>MSRLLALLALAPLLAGAAETTAPKPPSAFTVEAQRRVEAELPFADRADFERADRGLIRRPERLLIRNPDGSVAWQLGGYDFLLDGKPRDSINPSLQRQALLNLKYGLFEVAEGIYQVRGFDLANITFIRGDSGWIVVDTLTTPATARAAYELVSRELGERPIRTVIYSHAHADHFGGVRGLVEPQQVASGAVQIIAPAGFMEAAIKENVLAGNAMMRRATYQYGTQLPKGPQGQVDMAIGKGLARGPLSLLAPTRLIEGEGEDLVLDGVPFTFQNTPGTESPAEMNIWLPRQKALLMAENVVGTLHNLYTLRGAEVRDALGWSKYINQALHRFGRQAEVMFAVHNWPRWGNAEIVEVLEKQRDLYGYLHDQTLHLANQGVTIGQVHNRLRLPPSLDQEWYDRGYHGSVSHNARAVLNRYLGYYDGNPATLDPLSPEDSAGRYVEYMGGAERLLEQARASYARGEYRWVVEVVNRLVFAEPDNRAARELQADALEQLGYQAENAGWRNSYLSAAYELRHGVPRDQPTMKAGSADALAAMDTGLLFD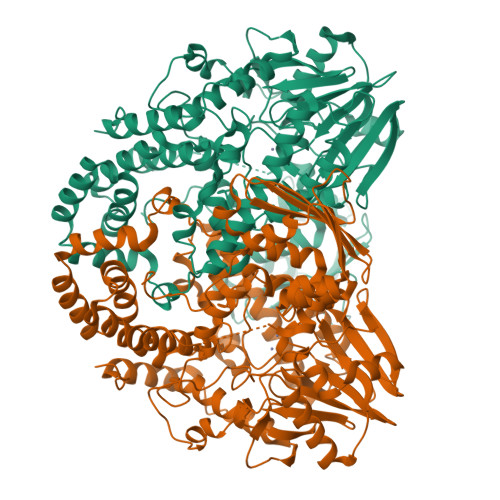YLGVRLDAGAAEGKALSINLRLPDIGENYLLELKNSHLNNLRGVQSEDAGQTVSIDRADLNRLLLKEVSAVRLVFEGKLKSSGNPLLLGQLFGMLGDFDFWFDIVTPAAKSEG[2x]> SRLSPIVRRARQYIQKHFSQSDLTLESVAEFLNVSPVYLSRMIKQELGISFIHLLTKIRMEKAAELLLSTELPIHEIAERVGYDTQH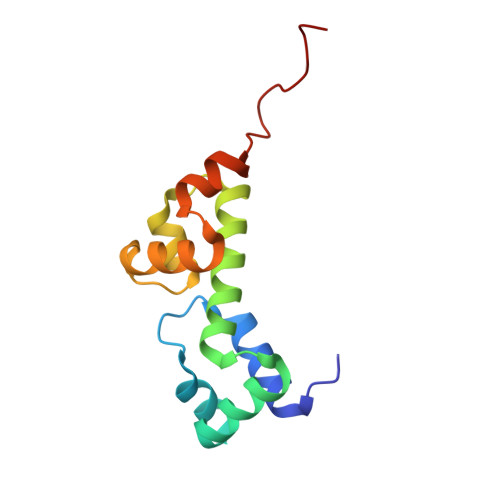YFSTAFKKAMGVSPNQYRRTRMISEYTDHHHHHH>[2x]HMLITD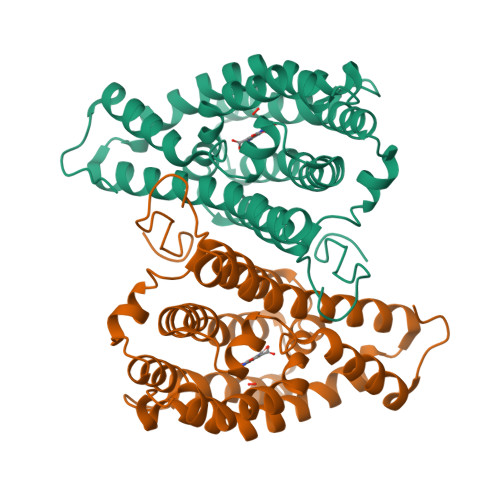TLSPQAFEEALRAKGDFYHIHHPYHIAMHNGDATRKQIQGWVANRFYYQTTIPLKDAAIMANCPDAQTRRKWVQRILDHDGSHGEDGGIEAWLRLGEAVGLSRDDLLSERHVLPGVRFAVDAYLNFARRACWQEAACSSLTELFAPQIHQSRLDSWPQHYPWIKEEGYFYFRSRLSQANRDVEHGLALAKAYCDSAEKQNRMLEILQFKLDILWSMLDAMTMAYALQRPPYHTVTDKAAWHTTRLVLEH>MVGQIAKEMGLRAYIVGGVVRDILLGKEVWDVDFVVEGNAIELAKELARRHGVNVHPFPEFGTAHLKIGKLKLEFATARRETYPRPGAYPKVEPASLKEDLIRRDFTINAMAISVNLEDYGTLIDYFGGLRDLKDKVIRVLHPVSFIEDPVRILRALRFA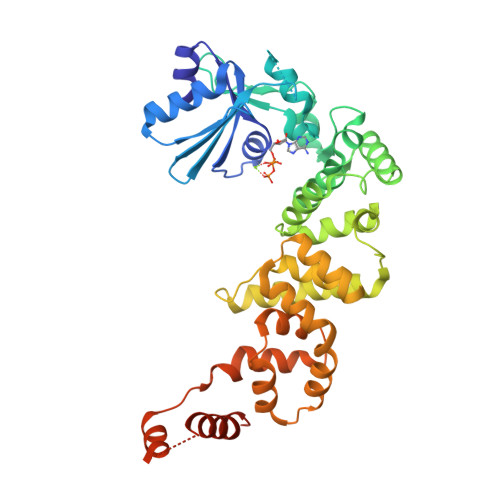GRLNFKLSRSTEKLLKQAVNLGLLKEAPRGRLINEIKLALREDRFLEILELYRKYRVLEEIIEGFQWNEKVLQKLYALRKVVDWHALEFSEERIDYGWLYLLILISNLDYERGKHFLEEMSAPSWVRETYKFMKFKLGSLKEELKKAKENYEVYRLLKPLHTSVLLLLMLEEELKEKIKLYLEKLRKVKLPKEKIEELKKQGLKGKELGERIEELKREIMNKIKLAAALEHHHHHH[2x]>[6x]GMASTTKSENVGAHIALFPCAGMGHLLPF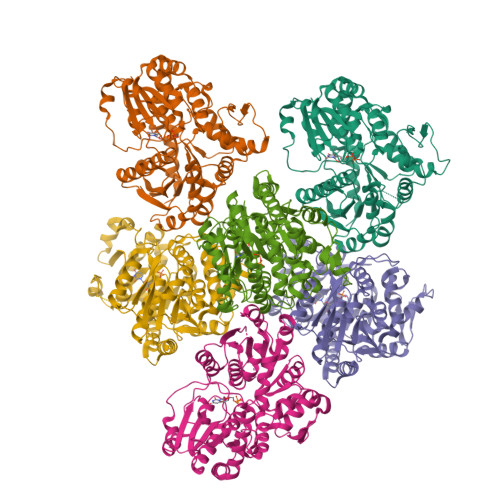LRLAAMLDARGCAVTVITVKPTVSAAESDHLSAFFTIHPRITRLEFQLLPYQKSGLRNDDPFFIQMETIATSVHLLRPLLSSLSPPLSAIVSDFTLTSQVTDLVSDLPISTYTLMTSSAAFFCLMAYLPKLLQIDVANRDAIEIPDLGPISMSSIPPKMLDPSDFFSAFISSNVSSLHKVKGVLINTFNSFESEAIEAVRRNGVDHILPIGPLESYDAKKAHDLPWLDEQPPESVLFVSFGSRTALSKEQIRELGAALEKSGCRFLWVLKGGKVDKEDKEEVEDMLGASFVERTKKKGLIVKGWVKQEQILAHPAIGGFVSHCGWNSVIEAARLGVPVLAWPQHGDQSVNAGVVEKAGLGLWVREWGWGQTKLIGREEIAEKMIEVMQDEKLRVSAGEVRAKAKETREVDGDSEALLQRLIHSFNNITQNS> MNQNLLVTKRDGSTERINLDKIHRVLDWAAEGLHNVSISQVELRSHIQFYDGIKTSDIHETIIKAAADLISRDAPDYQYLAARLAIFHLRKKAYGQFEPPALYDHVVKMVEMGKYDNHLLEDYTEEEFKQMDTFIDHDRDMTFSYAAVKQLEGKYLVQNRVTGEIYESAQFLYILVAACLFSNYPRETRLQYVKRFYDAVSTFKISLPTPIMSGVRTPTRQFSSCVLIECGDSLDSINATSSAIVKYVSQRAGIGINAGRIRALGSPIRGGEAFHTGCIPFYKHF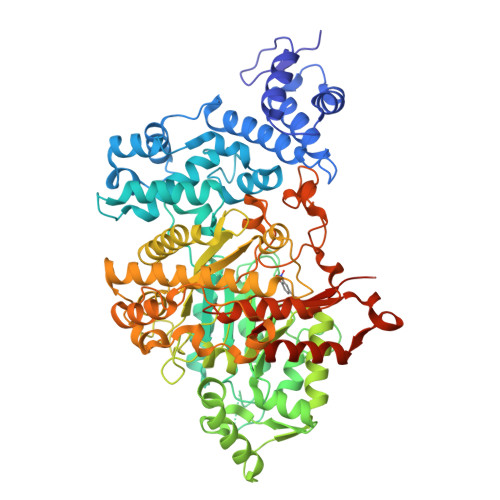QTAVKSCSQGGVRGGAATLFYPMWHLEVESLLVLKNNRGVEGNRVRHMDYGVQINKLMYTRLLKGEDITLFSPSDVPGLYDAFFADQEEFERLYTKYEKDDSIRKQRVKAVELFSLMMQERASTGRIYIQNVDHCNTHSPFDPAIAPVRQSNLCLEIALPTKPLNDVNDENGEIALCTLSAFNLGAINNLDELEELAILAVRALDALLDYQDYPIPAAKRGAMGRRTLGIGVINFAYYLAKHGKRYSDGSANNLTHKTFEAIQYYLLKASNELAKEQGACPWFNETTYAKGILPIDTYKKDLDTIANEPLHYDWEALRESIKTHGLRNSTLSALMPSETSSQISNATNGIEPPRGYVSIKASKDGILRQVVPDYEHLHDAYELLWEMPGNDGYLQLVGIMQKFIDQSISANTNYDPSRFPSGKVPMQQLLKDLLTAYKFGVKTLFYQNTRDGAEDAQDDLVPSIQDDGCESGACKI>[2x]SNAMSDMKHSKLLILGSGPAGYTAAVYAARANLNPVLITGMQQGGQLTTTTEVENWPGDPEGLTGPGLMDRMKEHAERFETEIIFDHINEVDFSTRPFVLKGDAASYSCDALIISTGASAKYLGLESEEAFKGRGVSACATCDGFFYRNQKVAVVGGGNTAVEEALYLSNIAAEVHLIHRRDSFRAEKILINRLMDKVQNGNIVLHTDRVLDEVLGDEMGVTGVRLKDVKTGGTEELDVMGAFIAI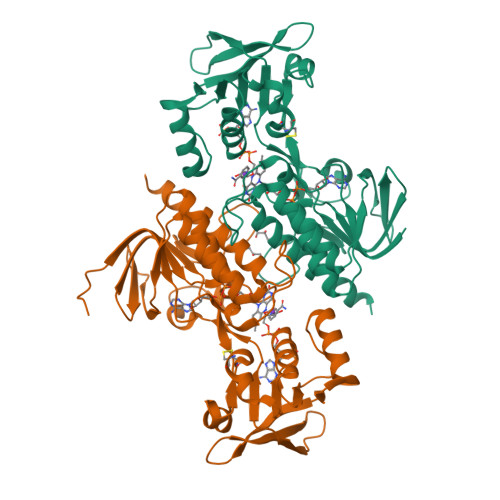GHSPNTQIFQGQLDMKDGYILVKSGLEGNATQTSVEGIFAAGDVMDHNYRQAITSAGTGCMAALDAERYLDSLNDK>GPGSMKVEKVFFVTSPIYYVNAAPHIGHVYSTLITDVIGRYHRVKGERVFALTGTDEHGQKVAEAAKQKQVSPYDFTTAVAGEFKKCFEQMDYSIDYFIRTTNEQHKAVVKELWTKLEQKGDIYLGRYEGWYSISDESFLTPQNITDGVDKDGNPCKVSLESGHVVTWVSEENYMFRLSAFRERLLEWYHANPGCIVPEFRRREVIRAVEKGLPDLSVSRARATLHNWAIPVPGNPDHCVYVWLDALTNYLTGSRLRVDESGKEVSLVDDFNELERFPADVHVIGKDILKFHAIYWPAFLLSAGLPLPKKIVAHGWWTKDRKKISKSLGNVFDPVEKAEEFGYDALKYFLLRESGFSDDGD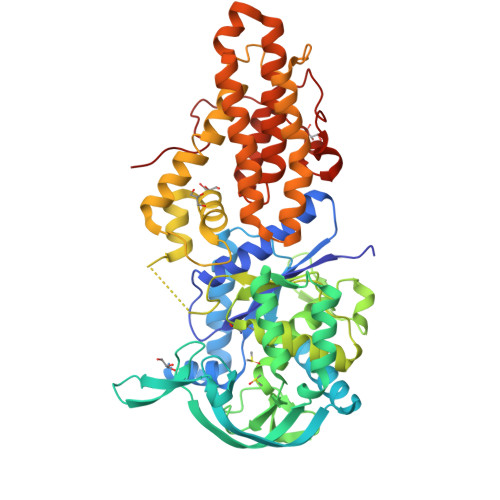YSDKNMIARLNGELADTLGNLVMRCTSAKINVNGEWPSPAAYTEEDESLIQLIKDLPGTADHYYLIPDIQKAIIAVFDVLRAINAYVTDMAPWKLVKTDPERLRTVLYITLEGVRVTTLLLSPILPRKSVVIFDMLGVPEVHRKGIENFEFGAVPPGTRLGPAVEGEVLFSKRST[2x]>GHMPAYVFSKESFLKFLEGHLEDDVVVVVSSDVTDFCKKLSESMVGEKEYCFAEFAFPADIFDAD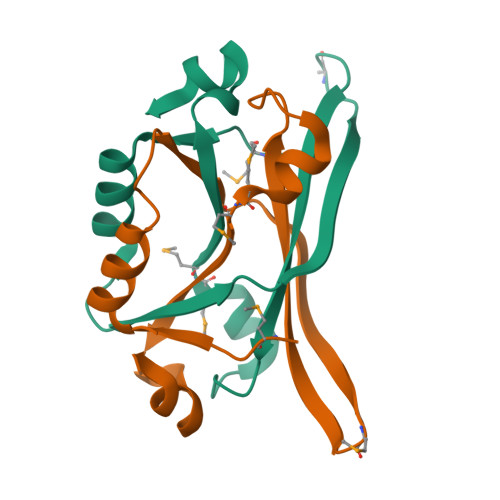EDEIDEMMKYAIVFVEKEKLSEAGRNAIR[2x]> GAMARVTMNEFEYLKLLGKGTFGKVILVKEKATGRYYAMKILKKEVIVAKDEVAHTLTENRVLQNSRHPFLTALKYSFQTHDRLCFVMEYANGGELFFHLSRERVFSEDRARFYGAEIVSALDYLHSEKNVVYRDLKLENLMLDKDGHIKITDFGLCKEGIKDGATMKTFCGTPEYLAPEVLEDNDYGRAVDWWGLGVVMYEMMCGRLPFYNQDHEKLFELILMEEIRFPRTLGPEAKSLLSGLLKKDPKQRLGGGSEDAKEIMQHRFFAGIVWQHVYEKKLSPPFKPQVTS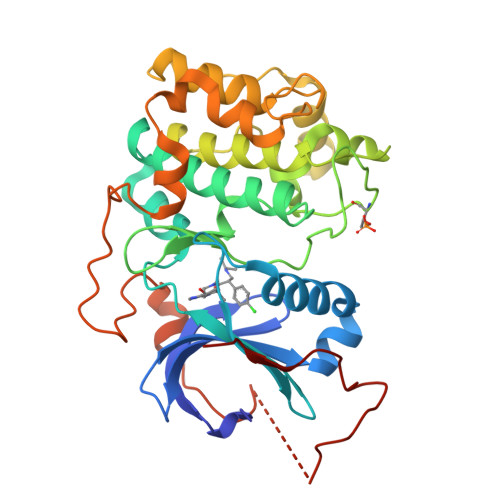ETDTRYFDEEFTAQMITITPPDQDDSMECVDSERRPHFPQFDYSASSTA> MAAIDKLVKASHLIDMNDIIREGNPTLRKVAEEVTFPLSEKEEILGEKMMQFLKHSQDPIMAEKLGLRGGVGLAAPQLDISKRIIAVLVPNVEDAQGNPPKEAYSLQEVMYNPKVVSHSVQDAALSDGEGCLSVDREVPGYVVRHARVTIEYFDKTGEKHRLKLKGYNSIVVQHEIDHIDGIM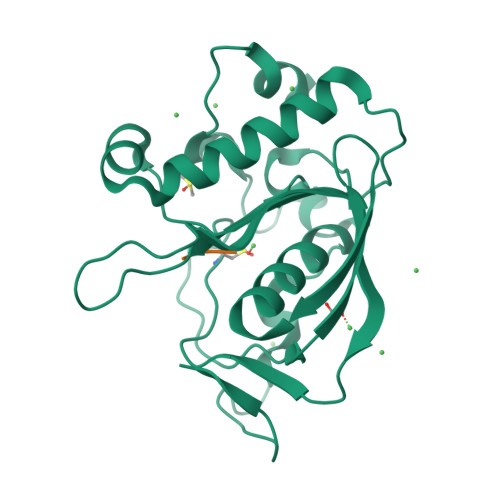FYDRINEKNPFAVKEGLLILE;> MAR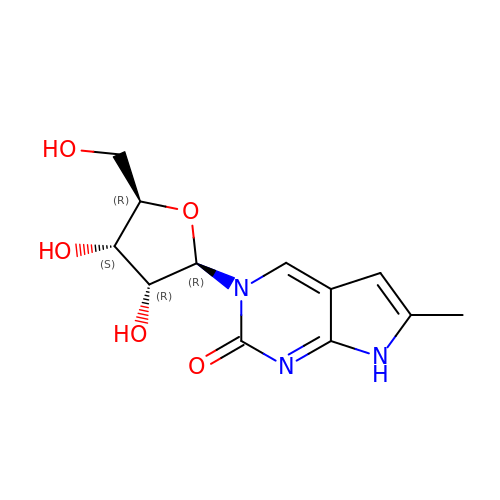6-methyl-3-(beta-D-ribofuranosyl)-3,7-dihydro-2H-pyrrolo[2,3-d]pyrimidin-2-one | C12 H15 N3 O5 | GCNYJWODKQPZDE-TURQNECASA-N>KVPVVGIVAALLPEMGIGFQGNLPWRLAKEMKYFREVTTLTNDNSKQNVVIMGRKTWESIPQKFRPLPKRINVVVSRSFDGELRKVEDGIYHSNSLRNCLTALQSSLANENKIERIYIIGG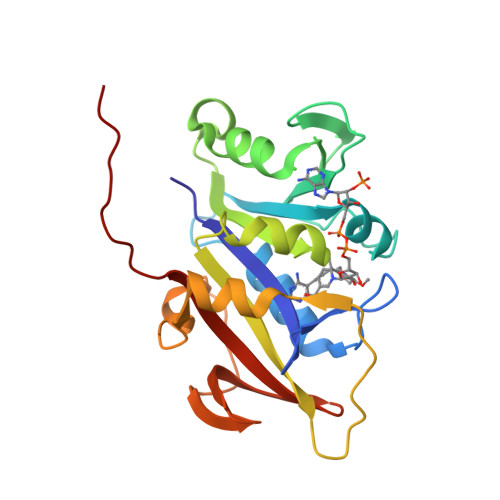GEIYRQSMDLADHWLITKIMPLPETTIPQMDTFLQKQELEQRFYDNSDKLVDFLPSSIQLEGRLTSQEWNGELVKGLPVQEKGYQFYFTLYTKKLEHHHHHHHH[2x]>MKPTMALKPLVFALAALMAVAAQAGPAEKWKPTPAPTGTVAAAVTDTQVSKDNKFDDTKTLNNAGANGSLSNSKGNLGANIAAGSGNQQDNAAAITSSAGDAATVFAVADIYQESKDNKFTNKGTQN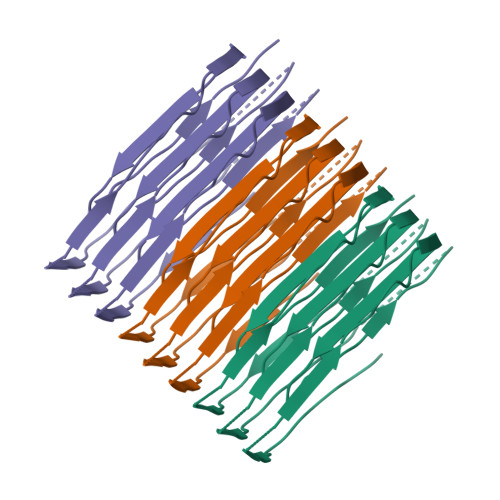NALLNNSANNSSGNVGVNVAAGQGNQQKNNLAIVTADGKNVAAASNTEQVSLDNHFLNEASSKHSYKPQYVVNNAGLLNSANNASGNIGVNVAAGAGNQQSNTLTLGSGCTVCAAGTGSKLAF[3x]> MKAYLGLYTARLETPARSLKEKRALIKPALERLKARFPVSAARLYGLDAWGYEVVGFTLLGNDPAWVE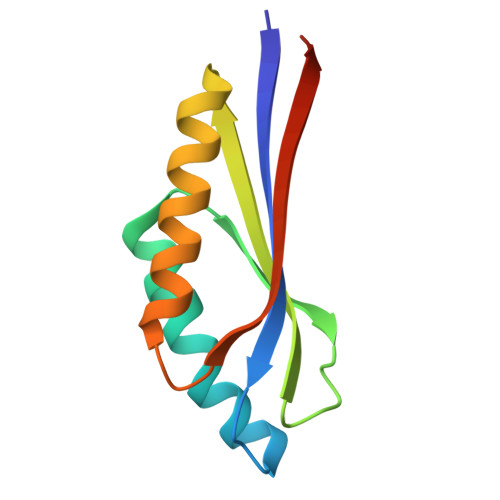ETMRAAARFLAEAGGFQVALEEFRLEAFELDGLL>GAMEVMNRETYKMDWSYSNSKQREIKTEIIKTASGSIAYCLTPDLRSPNGEDLPEMGKTSDAVYRVLLNGYPQKGPSELGVATTEEAHYATQLAVWIAANELTEEDLVAKNERVHNLMKRLVEASKKETGSQDVFFKVNPVDSQTATQNGDYLETGFYAVQTNAVSGSYTILPENAPKGLRIVNENGEEKSTLSINEKFKILLPKDTSSGNFKMKVKSTLTNLQAIAFKGSEKVQNTTVLLQRNSEKISTDLVVNWESVGSLKIMKLGEKKEVLKGAVFEVSNENFKQNVTTSDKGIAELGNLPIGIYSVKEIQAPAGYVLDRSVKKIEVKTGETAVLELKNENVKGELEITKVDVADGNTKLPNAEFTIYNEQGKEVVKGKTDEKGVAKFKLPYGKYTYKETIAPNGYVINEETFAFEIKENGEIIKHIVQDKKVEGELEITKVDVADGNTKLPNAEFTIYNEQGKEVVKGKTNEQGIAKFKL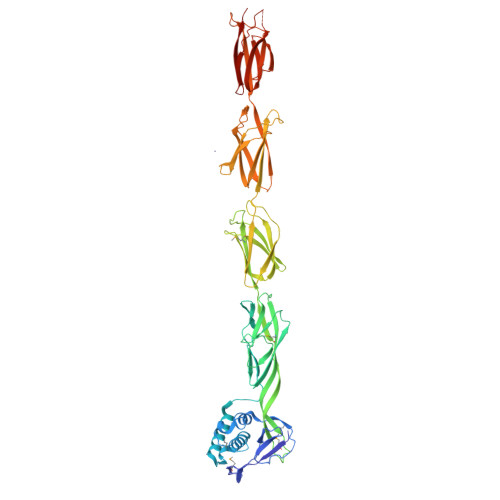PYGKYTYKETIAPNGYVINEEKFGFEIKENGEIIKHIVKNKK[2x]> GSNPNYCFAGKTSSISDLKEVPRKNITLIR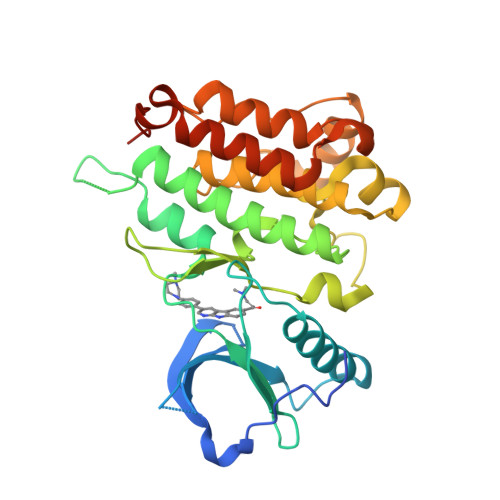GLGHGAFGEVYEGQVSGMPNDPSPLQVAVKTLPEVCSEQDELDFLMEALIISKFNHQNIVRCIGVSLQSLPRFILLELMAGGDLKSFLRETRPRPSQPSSLAMLDLLHVARDIACGCQYLEENHFIHRDIAARNCLLTCPGPGRVAKIGDFGMARDIYRASYYRKGGCAMLPVKWMPPEAFMEGIFTSKTDTWSFGVLLWEIFSLGYMPYPSKSNQEVLEFVTSGGRMDPPKNCPGPVYRIMTQCWQHQPEDRPNFAIILERIEYCTQDPDVINTALPIEYGPLVEEEEKV> STLEIAGLVRKNLVQFGVGEKNGSVRWVMNALGVKDDWLLVPSHAYKFEKDYEMMEFYFNRGGTYYSISAGNVVIQSLDVGFQDVVLMKVPTIPKFRDITQHFIKKGDVPRALNRLATLVTTVNGTPMLISEGPLKMEE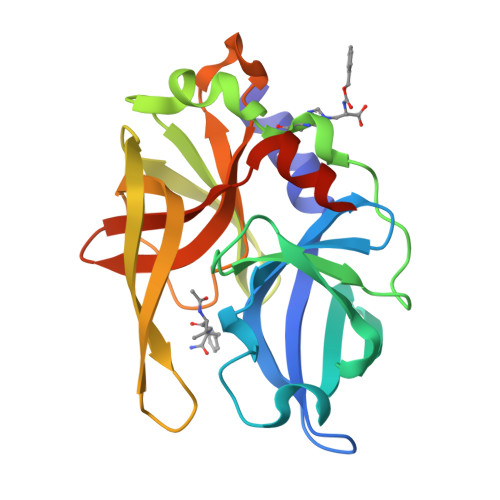KATYVHKKNDGTTVDLTVDQAWRGKGEGLPGMCGGALVSSNQSIQNAILGIHVAGGNSILVAKLVTQEMFQNIDKKIESQ> MPFPVTTQGSQQTQPPQKHYGITSPISLAAPKETDCLLTQKLVETLKPFGVFEEEEELQRRILILGKLNNLVKEWIREISESKNLPQSVIENVGGKIFTFGSYRLGVHTKGADIDALCVAPRHVDRSDFFTSFYDKLKLQEEVKDLRAVEEAFVPVIKLCFDGIEIDILFARLALQTIPE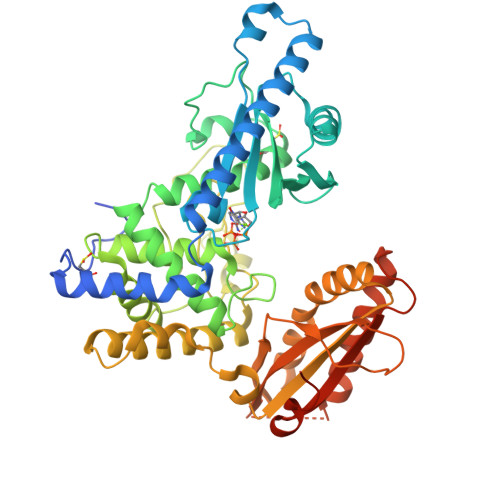DLDLRDDSLLKNLDIRCIRSLNGCRVTDEILHLVPNIDNFRLTLRAIKLWAKRHNIYSNILGFLGGVSWAMLVARTCQLYPNAIASTLVHKFFLVFSKWEWPNPVLLKQPEECNLNLPVWDPRVNPSDRYHLMPIITPAYPQQNSTYNVSVSTRMVMVEEFKQGLAITDEILLSKAEWSKLFEAPNFFQKYKHYIVLLASAPTEKQRLEWVGLVESKIRILVGSLEKNEFITLAHVNPQSFPAPKENPDKEEFRTMWVIGLVFKKTENSENLSVDLTYDIQSFTDTVYRQAINSKMFEVDMKIAAMHVKRKQLHQLLPSHVLQKKKKHSTEGVK>MAKAVDAAAAAAAAIAPVDTTVVNEDVALVENETCNDQNVQFDSLPSMKYASFLNSDGSVAIHAGERLGRGIVTDAITTPVVNTSAYFFNKTSELIDFKEKRRASFEYGRYGNPTTVVLEEKISALEGAESTLLMASGMCASTVMLLALVPAGGHIVTTTDCYRKTRIFIETILPKMGITATVIDPADVGALELALNQKKVNLFFTESPTNPFLRCVDIELVSKLCHEKGALVCIDGTFATPLNQKALALGADLVLHSATKFLGGHNDVLAGCISGPLKLVSEIRNLHHILGGALNPNAAYLIIRGMKT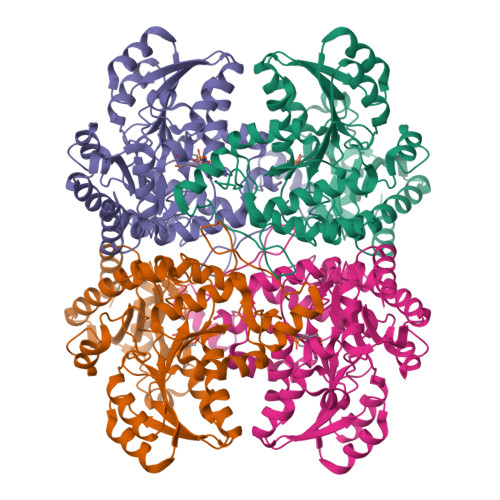LHLRVQQQNSTALRMAEILEAHPKVRHVYYPGLQSHPEHHIAKKQMTGFGGAVSFEVDGDLLTTAKFVDALKIPYIAPSFGGCESIVDQPAIMSYWDLSQSDRAKYGIMDNLVRFSFGVEDFDDLKADILQALDSI[12x]> MEEAELAYLLGELAYKLGEYRIAIRAYRIALKRDPNNAEAWYNLGNAYYKQGRYREAIEYYQKALELDPNNAEAWYNLGNAYYERGEYEEAIEYYRKALRLDPNN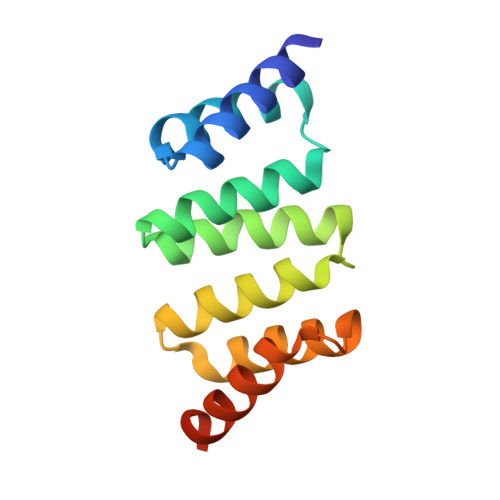ADAMQNLLNAKMREELEHHHHHH>[4x]MHFETTKDGFTIAIGNRIILSHSPDKPAFFAGFGEERMDMYRGNFDIEDYVIERTALRHAEVSGDSVTLSSAPGQAPRLRLTLDGNAIRLTALDETINRLWLRVVAETDEHVWGGGEQMSYFDMRGRRFPLWTSEPGVGRDKTTEITFKSDVSGKAGGDYYNTNYPQPTWL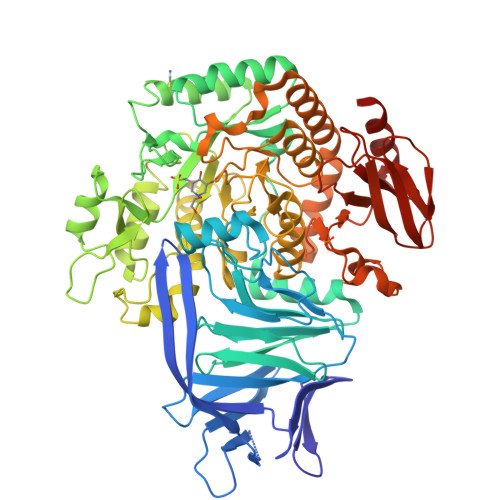SSRKYALHVETSAYSVFDFRNGDFHEIEIWAVPEKIEFFAGDSFADIVSALSLHFGRQPELPDWVYNGAIIGLKDGVNSFARLEKIRAAGTKVSGLWCEDWVGLRQTSFGARLFWDWQANDTRYPHLRQKIAELADQGIRFLGYVNPYLCVDGPLFPVAESAGYFATDVDGKTALVDFGEFDCGVVDFTNPAAADWFAAAIIGKNMLDFGLSGWMADFGEYLPIDIKLSNGVDAKLMHNAWPTLWAEVNAKGVESRGKTGEALFFMRAGFTGVQAHCPLIWGGDQSVDFSRHDGLVTVICGALSSGLMGNAYHHSDIGGYTSLFGNVRTAELIMRWTEMAAFTPVMRTHEGNRPRDNLQIDQDETVLAHFARMTAIYVALAPYLKSLSAEAAKTGLPVQRPLFLHYENEPQTYAVQDCYLYGADMLVAPVWKAGETQRSLYLPGHGEWVHLWSGKRHAGGRDITVETPLGEPAVFYRADSSHHRLFEQLRTIGLEHHHHHH> MHHHHHHGSLVPRGSMDYKDDDDKENLYFQGSRKKIFKPEELRQALMPTLEALYRQDPESLPFRQPVDPQLLGIPDYFDIVKNPMDL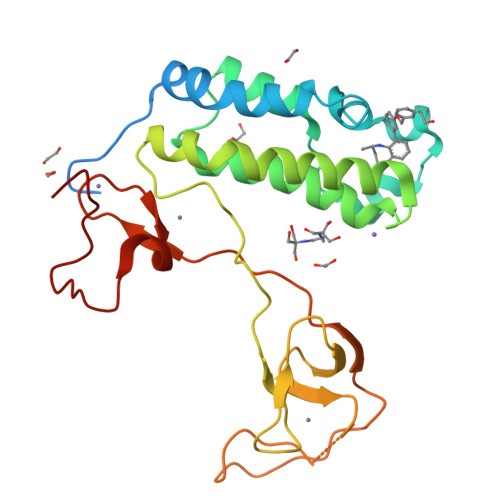STIKRKLDTGQYQEPWQYVDDVWLMFNNAWLYNRKTSRVYKFCSKLAEVFEQEIDPVMQSLGYCCGRKYEFSPQTLCCYGKQLCTIPRDAAYYSYQNRYHFCEKCFTEIQGENVTLGDDPSQPQTTISKDQFEKKKNDTLDPEPFVDCKECGRKMHQICVLHYDIIWPSGFVCDNCL>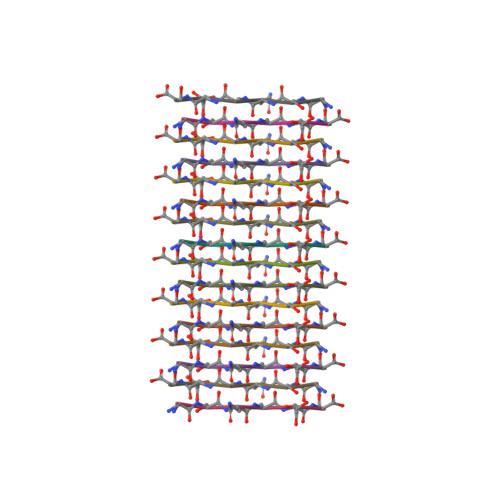 GSQASS>[2x]MAAPVVAPPGVVVSRANKRSGAGPGGSGGGGARGAEEEPPPPLQAVLVADSFDRRFFPISKDQPRVLLPLANVALIDYTLEFLTATGVQETFVFCCWKAAQIKEHLLKSKWCRPTSLNVVRIITSELYRSLGDVLRDVDAKALVRSDFLLVYGDVISNINITRALEEHRLRRKLEKNVSVMTMIFKESSPSHPTRCHEDNVVVAVDSTTNRVLHFQKTQGLRRFAFPLSLFQGSSDGVEVRYDLLDCHISICSPQVAQLFTDNFDYQTRDDFVRGLLVNEEILGNQIHMHVTAKEYGARVSNLHMYSAVCADVIRRWVYPLTPEANFTDSTTQSCTHSRHNIYRGPEVSLGHGSILEENVLLGSGTVIGSNCFITNSVIGPGCHIGDNVVLDQTYLWQGVRVAAGAQIHQSLLCDNAEVKERVTLKPRSVLTSQVVVGPNITLPEGSVISLHPPDAEEDEDDGEFSDDSGADQEKDKVKMKGYNPAEVGAAGKGYLWKAAGMNMEEEEELQQNLWGLKINMEEESESESEQSMDSEEPDSRGGSPQMDDIKVFQNEVLGTLQRGKEENISCDNLVLEINSLKYAYNISLKEVMQVLSHVVLEFPLQQMDSPLDSSRYCALLLPLLKAWSPVFRNYIKRAADHLEALAAIEDFFLEHEALGISMAKVLMAFYQLEILAEETILSWFSQRDTTDKGQQLRKNQQLQRFIQWLKEAEEESSEDD;>[2x]MPGSAAKGSELSERIESFVETLKRGGGPRSSEEMARETLGLLRQIITDHRWSNAGELMELIRREGRRMTAAQPSETTVGNMVRRVLKIIREEYGRLHGRSDESDQQESLHKLLTSGGLNEDFSFHYAQLQSNIIEAINELLVELEGTMENIAAQALEHIHSNEVIMTIGFSRTVEAFLKEAARKRKFHVIVAECAPFCQGHEMAVNLSKAGIETTVMTDAAIFAVMSRVNKVIIGTKTILANGALRAVTGTHTLALAAKHHSTPLIVCAPMFKLSPQFPNEEDSFHKFVAPEEVLPFTEGDILEKVSVHCPVFDYVPPELITLFISNIGGNAPSYIYRLMSELYHPDDHVL;>MAAVAVAVREDSGSGMKAELPPGPGAVGREMTKEEKLQLRKEKKQQKKKRKEEKGAEPETGSAVSAAQCQVGPTRELPESGIQLGTPREKVPAGRSKAELRAERRAKQEAERALKQARKGEQGGPPPKASPSTAGETPSGVKRLPEYPQVDDLLLRRLVKKPERQQVPTRKDYGSKVSLFSHLPQYSRQNSLTQFMSIPSSVIHPAMVRLGLQYSQGLVSGSNARCIALLRALQQVIQDYTTPPNEELSRDLVNKLKPYMSFLTQCRPLSASMHNAIKFLNKEITSVGSSKREEEAKSELRAAIDRYVQEKIVLAAQAISRFAYQKISNGDVILVYGCSSLVSRILQEAWTEGRRFRVVVVDSRPWLEGRHTLRSLVHAGVPASYLLIPAASYVLPEVSKVLLGAHALLANGSVMSRVGTAQLALVARAHNVPVLVCCETYKFCERVQTDAFVSNELDDPDDLQCKRGEHVALANWQNHASLRLLNLVYDVTPPELVDLVITELGMIPCSSVPVVLRVKSSDQ[2x];>[2x]MDDKELIEYFKSQMKEDPDMASAVAAIRTLLEFLKRDKGETIQGLRANLTSAIETLCGVDSSVAVSSGGELFLRFISLASLEYSDYSKCKKIMIERGELFLRRISLSRNKIADLCHTFIKDGATILTHAYSRVVLRVLEAAVAAKKRFSVYVTESQPDLSGKKMAKALCHLNVPVTVVLDAAVGYIMEKADLVIVGAEGVVENGGIINKIGTNQMAVCAKAQNKPFYVVAESFKFVRLFPLNQQDVPDKFKYKADTLKVAQTGQDLKEEHPWVDYTAPSLITLLFTDLGVLTPSAVSDELIKLYL;>MEFQAVVMAVGGGSRMTDLTSSIPKPLLPVGNKPLIWYPLNLLERVGFEEVIVVTTRDVQKALCAEFKMKMKPDIVCIPDDADMGTADSLRYIYPKLKTDVLVLSCDLITDVALHEVVDLFRAYDASLAMLMRKGQDSIEPVPGQKGKKKAVEQRDFIGVDSTGKRLLFMANEADLDEELVIKGSILQKHPRIRFHTGLVDAHLYCLKKYIVDFLMENGSITSIRSELIPYLVRKQFSSASSQQGQEEKEEDLKKKELKSLDIYSFIKEANTLNLAPYDACWNACRGDRWEDLSRSQVRCYVHIMKEGLCSRVSTLGLYMEANRQVPKLLSALCPEEPPVHSSAQIVSKHLVGVDSLIGPETQIGEKSSIKRSVIGSSCLIKDRVTITNCLLMNSVTVEEGSNIQGSVICNNAVIEKGADIKDCLIGSGQRIEAKAKRVNEVIVGNDQLMEI[2x];>MNSQYMFDYPAINIDVRCHRLLSSVSYVAYNKFHTHDVSTYEHCEIPLEKLRLGFGRRNSLADFYSLGELPASWGPACYFSSVKPMMYTFQGMASDLSRFDLTSFSRKGLPNVLKALSWPLGIPDCEIFSICSDRFVRGLQTRDQLMSYILRMGDSHSLDECIVQAHKKILQEARRLGLSDEHYNGYDLFREIGSLVCLRLINAEPFDTASSGEALDVRTVIRSYRASDPSTGLTEYGNSLWTPIHSHVDENDESSSDSDFGSHHHHHH[2x]

Phosphorylated eIF2 (eIF2-P) inhibits translation by binding to eIF2’s dedicated, heterodecameric nucleotide exchange factor eIF2B and conformationally inactivating it. eIF2B is a twofold symmetric heterodecamer composed of two copies each of α, β, δ, γ, and ε subunits. eIF2B can exist in a range of stable subcomplexes (eIF2Bβδγε tetramers and eIF2Bα2 dimers) if the concentrations of its constituent subunits are altered. In this arrangement, eIF2α binding to eIF2B critically positions the GTPase domain in eIF2’s γ-subunit, allowing for efficient catalysis of nucleotide exchange. eIF2B’s catalytically active conformation (“A-State”) becomes switched to an inactive conformation upon eIF2-P binding (Inhibited or “I-State”), which displays altered substrate-binding interfaces. We here provide cellular, biochemical, and structural insight into this question, showing that the SFSV NSs evades all branches of the ISR by binding to eIF2B and selectively blocking eIF2-P binding, thereby maintaining eIF2B in its active A-State.

Refinement of this class resulted in a map with an average resolution of 2.6 Å. After docking the individual eIF2B subunits into the recorded density, we observed significant extra density next to both eIF2Bα subunits, indicating that two copies of NSs are bound to each eIF2B decamer. Interestingly, whereas eIF2α-P forms extensive interactions with both the α and the δ subunits of eIF2B, the NSs mainly interacts with the eIF2Bα subunit. Thus, despite binding to a region known to influence eIF2B’s conformation, an overlay of the NSs-bound eIF2B and apo eIF2B shows that the overall conformation of eIF2B in the two structures are virtually identical. By contrast, the eIF2B–NSs and eIF2B–eIF2α-P overlay shows major conformational differences. The surface of the N-terminal domain forms a hand shape that grips the alpha helices of eIF2Bα, akin to a koala grabbing a eucalyptus branch. In this arrangement, the N-terminal domain extends three loops that contact eIF2Bα. The first two loops sit in a groove between helices α3 and α4 and the third loop just below helix α3, effectively sandwiching helix α3. Together, the three loops extend five aromatic amino acids to contact eIF2Bα. In addition, the side chain of NSs H36 and the backbone carbonyl of NSs T35 both contact eIF2Bδ R321. NSs is an antagonist of eIF2B’s inhibitor eIF2-P, deploying an overlapping binding site. Whereas eIF2-P shifts eIF2B to its inactive I-State conformation by closing the angle between the eIF2Bα and eIF2Bδ subunits, NSs engages the enzyme to opposite effect, binding to an overlapping site with eIF2-P but preserving the angle between eIF2Bα and eIF2Bδ and locking it into its active A-State conformation.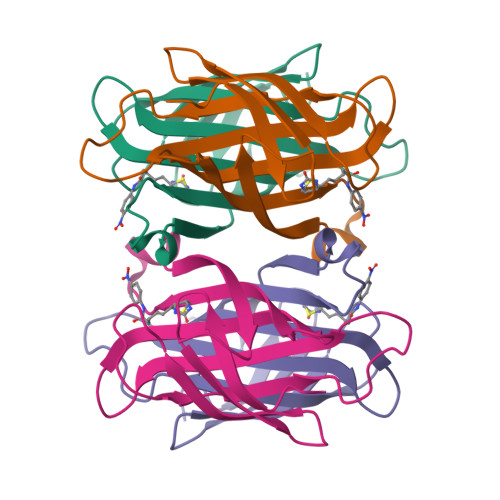>[2x]AEAGITGTWYNQLGSTFIVTAGADGALTGTYESAVGNAESRYVLTGRYDSAPATDGSGTALGWTVAWKNNYRNAHSATTWSGQYVGGAEARINTQWLLTSGTTEANAWKSTRVGHDTFTKVKPSAAS The Type-IV restriction endonuclease (REase)ScoA3McrA (abbreviated as ScoMcrA hereafter) catalyzes multiple double strand cleavages 16–28 nucleotides (nt) away from the phosphorothioate linkage with the core sequence GPSGCC/GPSGCC. The DNA PT-dependent REase ScoMcrA distinguishes PT-DNA from normal DNA which differs only by one oxygen-to-sulfur swap, and presumably encodes a domain to specifically recognize sulfur on PT-DNA. Each ScoMcrA protomer consists of a head domain, an uncharacterized domain, a SRA-like domain, and an HNH domain. The uncharacterized domain binds specifically to PT-DNA whose sulfur atom is in the Rp but not in the Sp configuration, therefore we named it sulfur-binding domain (SBD).

In contrast, the ScoMcrA‒SBD structure exists as a monomer. Although there are sulfur atoms in both strands of PT-DNA, which contain a palindromic GPSGCC core sequence, only one sulfur atom in PT-DNA is recognized by ScoMcrA-SBD in both structures. The sulfur atom on PT-DNA fits snugly in a cavity on the surface of SBD. The wall of this sulfur-binding cavity of SBD is lined with non-polar functional groups, including the β-methylene groups of Y164 and H116, the β-methyl group of A168, and the γ-methylene group of R117. The hydrophobic pyrolidine ring of P165 forms the bottom of this sulfur-binding cavity. Our structure reveals that the tip of the α9–α10 loop of ScoMcrA, whose sequence is S187RGRR191, inserts into the major groove of PT-DNA and provides base-specific contacts for the GPSGCC core sequence. At the center of this interface, the guanidinium group of R190 in the S187RGRR191 loop forms two hydrogen bonds with the O6 atoms of G3 and G4 of the G3PSG4C5C6/G6′G5′C4′C3′ core sequence (′ denotes bases on the complementary strand). On the other hand, upon binding of PT-DNA, the hydroxyphenyl group of the side-chain of Y164 is flipped open allowing the sulfur atom in PT-DNA to access the ScoMcrA-SBD cavity. Hence, the association with PT-DNA leads to a 98° rotation of the hydroxyphenyl group from Y164 side-chain. In comparison with the DNA strand that is not in contact with ScoMcrA-SBD, the sulfur atom in the SBD-bound strand of PT-DNA is rotated about the phosphodiester backbone by 80° outward so that it fits better into the ScoMcrA-SBD sulfur-binding cavity.

> GSREAPKTFHRRVGDVRPARRAMGPALHRPVLLLWAIGQAVARAPRLQPWSTTRDAVAPLMEKYGQVEDGVDGVRYPFWALVRDDLWCVEQAEELTLTSRGRRPTLESLNAVDPSAGLREDDYNLLRSQPEAAASAAAGLIARYFHLLPAGLLEDFGLHELLAGRWPDALRP> MNKHDAIQLI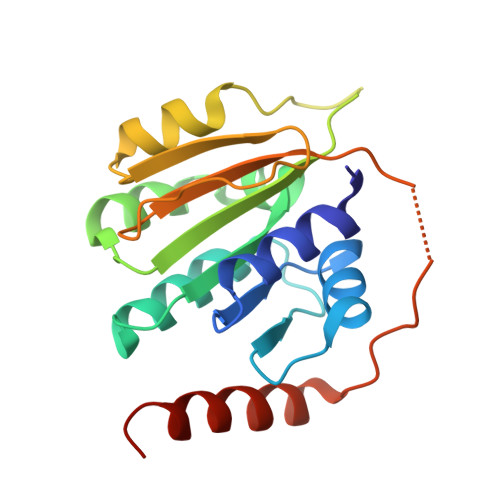LGQFPSAYLVSTCGHISRDLYNINDRARNFYMVGSMGMAAPVGLGLSTVYPDVPLVVLDGDGSFLMNMGIITMIGHQKPKNFIHVVLDNGMHESTGGQRTVPLVNVTDIALQVGYEYAIEINSGQKSFDLPNEGPGLIHIKVEPRSEKIGKRVHWTPQEIVQRFTNELTLENEVSV> TDQL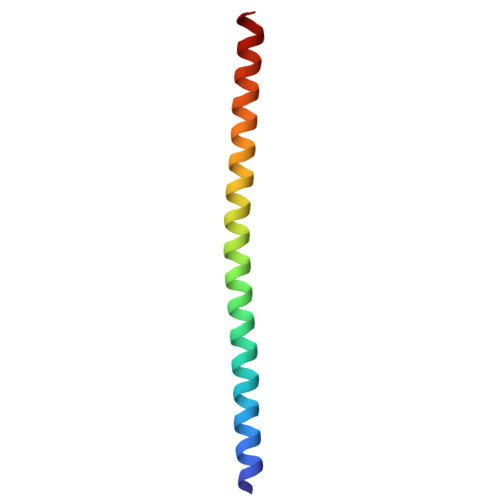KKAKAEAQVIIEQANKRRSQILDEAKAEAEQERTKIVAQAQAEIEAERKRAREELRK> GPGSMLLSMSQQVSLVATLIANPAKAALAPSLGIKASAAVNATGLYWLADDIACDIPLPL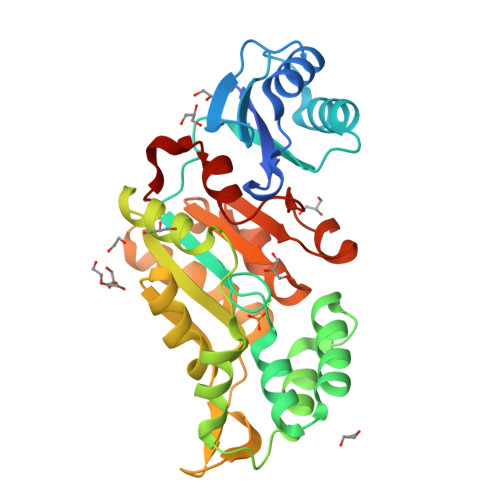GMEASEADASLRATLDGAPIDVVVQEQERRRKKILIADMDSTMIGQECIDELAEEAGLRDHVAAITARAMNGEIAFEPALRERVALLKGLPLSVIDKVISTRITLTPGGPQLVRTMRKHGAYTALVSGGFTSFTRRIAEMIGFNEERANRLIDDGTRLTGTVAEPILGREAKVEKLVEIAERVGLTPEDAIAVGDGANDLGMIQLAGTGVALHAKPAVAAQAKMRIDHGDLTALLYIQGYRKADFVQ> MTVDANAASSTTTTTDYYFDSYSHYGIHMEMLKDCHRTTSYRDAMWRNAYLFKDKVVLDVGCGTGILSMFAAKAGARKVIGVDCSTVAVQAREIVKDNGFEDVITIIQGKVEEIQLDEKVDIIISEWMGYFLLYESMLNTVLCARDNLGTPDVKMFPDKANMHVCGITDEQYIQERFNIWDNVQGIDFSYFKRLSFIEPLVDTVERSQIVT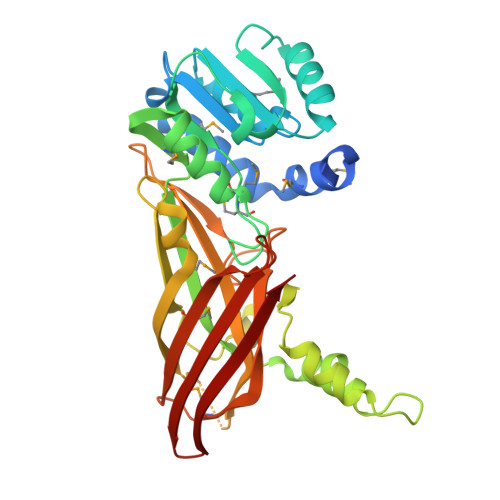NVAPLVSFDINTVKEADLSFTSEFALEAQASRGKRNGGNSIIYVHALSVHFDTPFTAGHEVVILDTTPYSPPTHWRQTVLYLFNPLRMRAGERATFRMKCSPNALNGRDLDISLHVDFEGALQISHYDQDFRLR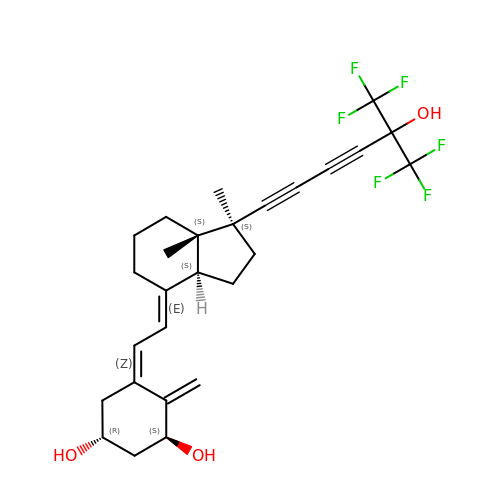(1~{R},3~{S},5~{Z})-5-[(2~{E})-2-[(1~{S},3~{a}~{S},7~{a}~{S})-1,7~{a}-dimethyl-1-[6,6,6-tris(fluoranyl)-5-oxidanyl-5-(trifluoromethyl)hexa-1,3-diynyl]-2,3,3~{a},5,6,7-hexahydroinden-4-ylidene]ethylidene]-4-methylidene-cyclohexane-1,3-diol | C27 H30 F6 O3 | MVLLQZOKYYYEBT-ZUDXOIQDSA-N>MIRNRLSELLSERGLKISRVAKDVKIARSSLTSMAQNDSEMIRYDAIDKLCSYLHISPSEFFEHNPINFDFTFDEEPNYKINDVFEGFEVTANITHAFSIENFDFEILVDVELDNRQKLNFDLDVSYKETEKITNSQHRFIFTIKNEDE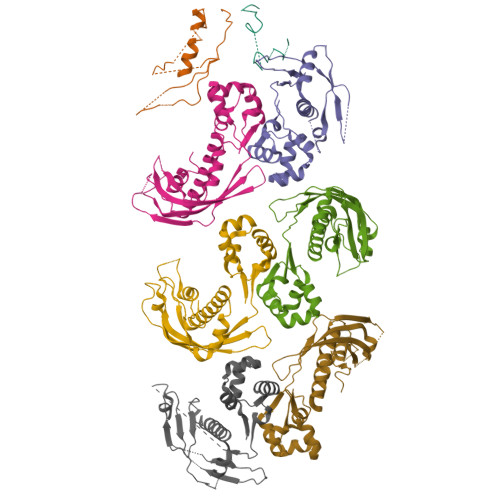NIGLKKYVDSLSAGLKNLLFKKINQKLSGYVSEIIVKNIDDIEELFPNKGEKSTTLHKEILQTDSRLSSDIFKEYLEHHHHHH[8x]> TETTSFSITKFGPDQQNLIFQGDGYTTKERLTLTKAVRNTVGRALYSSPIHIWDSK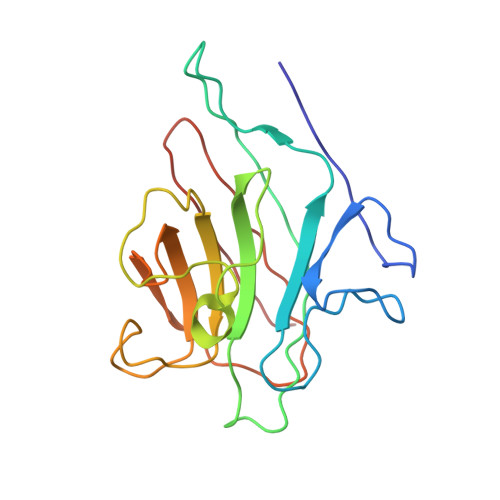TGNVANFVTSFTFVIDAPNSYNVADGFTFFIAPVDTKPQTGGGYLGVFNSKDYDKTSQTVAVEFDTFYNTAWDPSNGDRHIGIDVNSIKSINTKSWKLQNGKEANVVIAFNAATNVLTVSLTYPN(2R,4R,5R,6R,7R)-2,4,5,6,7-PENTAHYDROXY-2,8-BIS(PHOSPHONOOXY)OCTANOIC 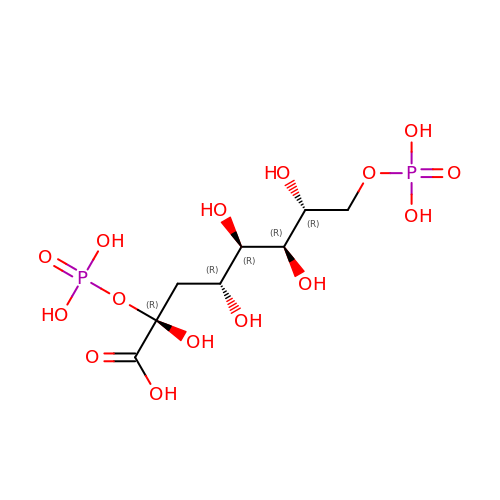ACID | C8 H18 O15 P2 | FGVVFQVXYXTAAW-HXUQBWEZSA-N>[8x]MQKPVCLVVAMTPKRGIGINNGLPWPHLTTDFKHFSRVTKTTPEEASRFNAVVMGRKTWESMPRKFRPLVDRLNIVVSSSLKEEDIAAEKPQAEGQQRVRVCASLPAALSLLEEEYKDSVDQIFVVGGAGLYEAALSLGVASHLYITRVAREFPCDVFFPAFPGDDILSNKSTAAEKDNEATYRPIFISKTFSDNGVPYDFVVLEKRRKTDDAATAEPSNAMSSLTSTRETTPVH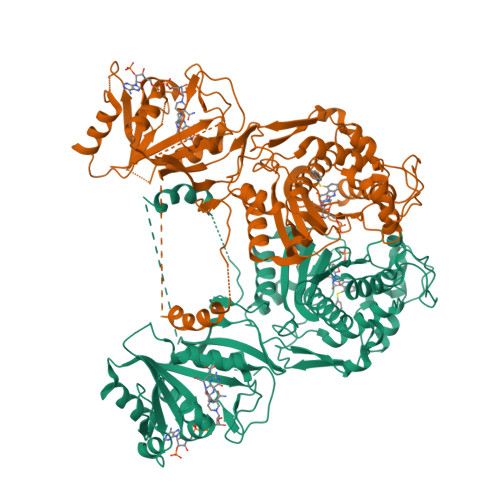GLQAPSSAAAIAPVLAWMDEEDRKKREQKELIRAVPHVHFRGHEEFQYLDLIADIINNGRTMDDRTGVGVISKFGCTMRYSLDQAFPLLTTKRVFWKGVLEELLWFIRGDTNANHLSEKGVKIWDKNVTREFLDSRNLPHREVGDIGPGYGFQWRHFGAAYKDMHTDYTGQGVDQLKNVIQMLRTNPTDRRMLMTAWNPAALDEMALPPCHLLCQFYVNDQKELSCIMYQRSCDVGLGVPFNIASYSLLTLMVAHVCNLKPKEFIHFMGNTHVYTNHVEALKEQLRREPRPFPIVNILNKERIKEIDDFTAEDFEVVGYVPHGRIQMEMAV> MDVDLPPPGPLTSGGLRVTALGGINEIGRNMTVFEHLGRLLIIDCGVLFPGHDEPGVDLILPDMRHVEDRLDDIEALVLTHGHEDHIGAIPFLLKLRPDIPVVGSKFTLALVAEKCREYRITPVFVEVREGQSTRHGVFECEYFAVNHSTPDALAIAVYTGAGTILHTGDIKFDQLPPDGRPTDLPGMSRLGDTGVDLLLCDSTNAEIPGVGPSESEVGPTLHRLIRGADGRVIVACFASNVDRVQQIIDAAVALGRRVSFVGRSMVRNMRVARQLGFLRVADSDLI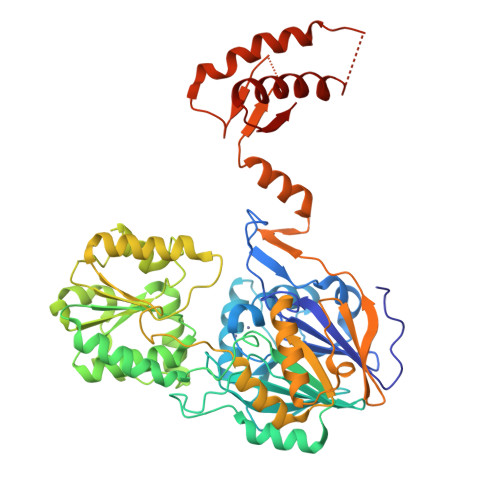DIAAAETMAPDQVVLITTGTQGEPMSALSRMSRGEHRSITLTAGDLIVLSSSLIPGNEEAVFGVIDALSKIGARVVTNAQARVHVSGHAYAGELLFLYNGVRPRNVMPVHGTWRMLRANAKLAASTGVPQESILLAENGVSVDLVAGKASISGAVPVGKMFVDGLIAGDVGDITLGERLILSSGFVAVTVVVRRGTGQPLAAPHLHSRGFSEDPKALEPAVRKVEAELESLVAANVTDPIRIAQGVRRTVGKWVGETYRRQPMIVPTVIEV> HMAALDSLSLFTSLGLSEQKARETLKNSALSAQLREAATQAQQTLGSTIDKATGILLYGLASRLRDTRRLSFLVSYIASKKIHTEPQLSAALEYVRSHPLDPIDTVDFERECGVGVIVTPEQIEEAVEAAINRHRPQLLVERYHFNMGLLMGEARAVLKWADGKMIKNEVDMQVLHLLGPKLEADLEKKFKVAKARLEETDRRTAKDVVENGETADQTLSLMEQLRGEALKFHKPGENYKTPGYVVTPHTMNLLKQHLEITGGQVRTRFPPEPNGILHIGHAKAINFNFGYAKANNGICFLRFDDTNPEKEEAKFFTAICDMVAWLGYTPYKVTYASDYFDQLYAWAVELIRRGLAYVCHQRGEELKGHNTLPSPWRDRPMEESLLLFEAMRKGKFSEGEATLRMKLVMEDGKMDPVAYRVKYTPHHRTGDKWCIYPTYDYTHCLCDSIEHITHSLCTKEFQARRSSYFWLCNALDVYCPVQWEYGRLNLHYAVVSKRKILQLVATGAVRDWDDPRLFTLTALRRRGFPPEAINNFCARVGVTVAQTTMEPHLLEACVRDVLNDTAPRAMAVLESLRVIITNFPAAKSLDIQVPNFPADETKGFHQVPFAPIVFIERTDFKEEPEPGFKRLAWGQPVGLRHTGYVIELQHVVKGPSGCVESLEVTCRRADAGEKPKAFIHWVSQPLMCEVRLYERLFQHKNPEDPTEVPGGFLSDLNLASLHVVDAALVDCSVALAKPFDKFQFERLGY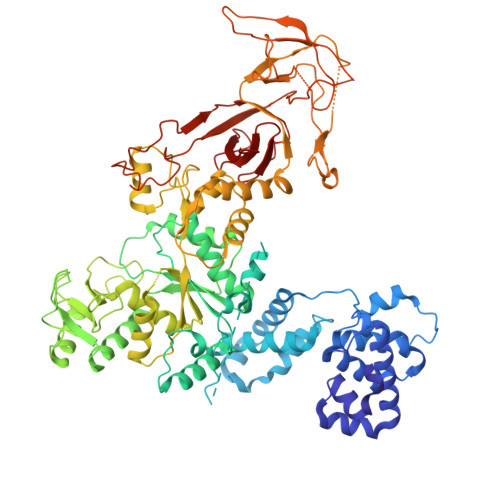FSVDPDSHQGKLVFNRTVTLKEDPGKV> GPLGSKLNDILHVYEKSKERELQSQ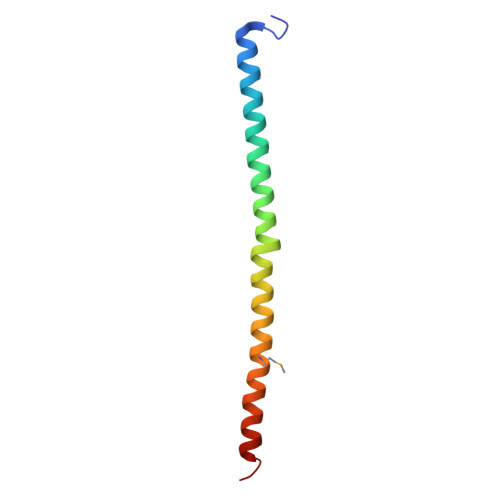LFNAWRNRFCFYTEECNIQAISKRNYQLEKMVLKKFRERLLEIVKSEE>MSKKTIVSMAVIRRLPRYHRYLEELLKNDVKRISSRELSEKMGVTASQIRQDLNNFGGFGQQGYGYNVEELYNNLTKILGLDK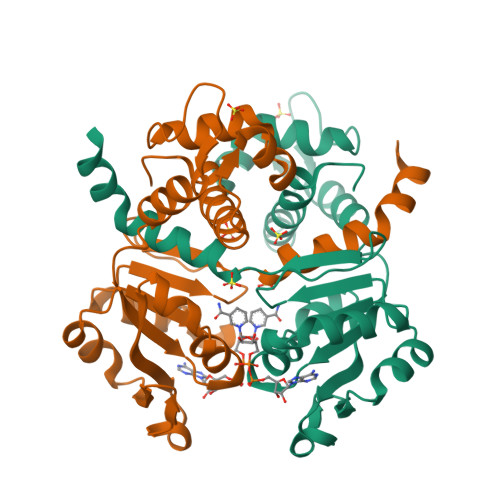TYNTIIIGAGNLGQAIANYTSFEKSGFNLKGIFDINPRLFGLKIRDVEVMDVETVEDFIARNKIDIGILCIPKDNAQYTADRLVRAGIKAIWNFLPIDLKVPDDVILENVHLSDSLFTVSYRLNEEELFKKLKGETAKIDG[2x]>[4x]MTVHSPRFDLRQYQREWFANPRKDVLAGIVVALALIPEAIAFSIIAGVDPQVGLYASF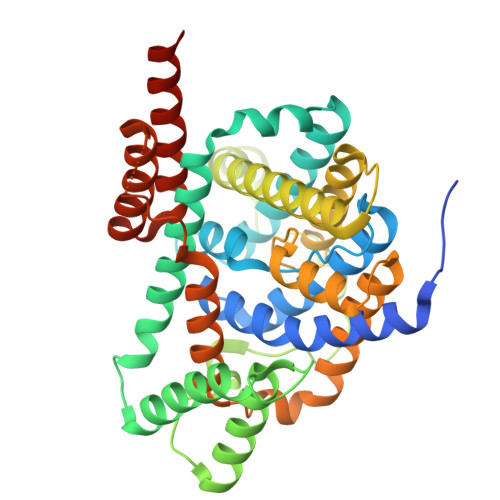IIALITAFLGGRPGMISAATGAMALLMTGLVKDHGIQYLFAATVLTGVLQVVFGWAKLARYLKFVPRSVMVGFVNALAILIFMAQLPQFVGANWQMYAMVAAGLAIIYLLPLVFKAMPSALVAIVVLTVVAVVTGADVKTVGDMGTLPTALPHFQFPQVPLTFETLAIIFPVALTLSLVGLLESLLTAQLIDERTDTTSDKNVESRGQGVANIVTGFFGGMAGCAMIGQSMINVTSGGRGRLSTFVAGAFLMVLILALQPLLVQIPMAALVAVMMVVAISTFDWGSLRTLTVFPKGETVVMLATVAVTVFTHDLSLGVLIGVVLSALFFARKVSQLSQVTPVD>MIERGKFRSLTLVNWNGFFARTFDLDELVTTLSGGNGAGKSTTMAAFVTALIPDLTLLHFRNTTEAGATSGSRDKGLHGKLRAGVCYSTLDVINSRHQRVVVGVRLQQVAGRDRKVDIKPFMIQGLPTAIQPTQLLTENVGERQARVLPLNELKDRLDEMEGVQFKQFNSITDYHAQMFDLGVIPKRLRSASDRSKFYRLIEASLYGGISSAITRSLRDYLLPENSGVRKAFQDMEAALRENRITLEAIRVTQSDRDLFKHLITEATSYVSADYMRHANERRTHLDEALALRGELFGSHKQLATEQYRHVEMARELAEQSGASSDLETDHQAASDHLNLVQTAMRQQEKIDRYQVDLEELSYRLEEQTDVVEEAGELQAEYEARTEATEQEVDELKSQLADYQQALDVQQTRAIQYQQALQALERARELCRLPDLSVDNAEEWLETFQAKEQQATEALLALEQKLSVADAAHNQFEQAYQLVKNIVGETSRSEAWQSARELLRDWPSQRHLADRVQPLRMRLSELEQRLNNQQNAERLLSEFCKRQGRQYQAEDLEALQNELEARQEALSLSVNEGGERRMEMRQELEQLKQKIQSLTARAPVWLAAQDTLNQLCEQSGETLASSNDVTEYMQQLLEREREATVERDEVAAQKRELEKQIERLSQPSGAEDSRMIALAERFGGVLLSEIYDDITIDDAPYFSALYGPARHGIVVPDLSLVRPHLETLEDCPEDLYLIEGDPQSFDDSVFNAEEQTNAVLVKSSDRQWRYSRYPELPLFGRAARENRLEALNLERDALAERYATLSFDVQKIQRAHQAFSQFVGKHLSVAFDTDPEAEIRELRQRHTELEREVSRFEDQTQQQRQQYAQAKESLTTLNRLIPQVTLLLDETLIDRVEEVREEMDEAQEAARFLQQHGSALTKLEPMVAVLQSDPQQHEQLQQDYETAKHSQHQAKQQAFALVEIVQRRVHFSYSDSAGMLSENADLNDKLRQRLEHAESDRSRAREQLRQQQAQYSQFNQVLASLKSSYETKQDMLKELLQEMKDIGVQADANAEMRARERRDRLHEALSVNRSRVNQLEKQIAFCEAEMENVQKKLRKLERDYYQIREQVVSAKAGWCAVMRMVKDNGVERRLHRRELAYMEGGALRSMSDKALGALRLAVADNEHLRDALRLSEDPKRPERKVQFFIAVYQHLRERIRQDIIRTDDPVDAIEQMEIELARLTEELTAREQKLAISSKSVANIIRKTIQREQNRIRMLNQGLQAVSFGQVRGVRLNVNVRESHAILLDVLSEQQEQHQDLFNSQRLTFSEAMAKLYQRLNPQVDMGQRLPQTIGEELLDYRNYLELDVEVNRGSDGWLKAESGALSTGEAIGTGMSILVMVVQSWEEESRRLRGKDISPCRLLFLDEAARLDAKSIATLFELCERLQMQLIIAAPENISPEKGTTYKLVRKVFKNHEHVHVVGLRGFGQDAPATQLISDVTA[2x];>MSEYSQTVPELVSWARKNDFSISLPVERLAFLMAIAVLNSERLDGEMSEGELIDAFREVCKGFEQTAESVAVRANNAINDMVRQKLLNRFTSELADGNAIYRLTPLGISISDYYIRQREFSTLRLSMQLSIVANELHRAAEAAEEGGDEFHWHRNVFAPLKYSVAEIFDSIDMSQRLMDEQQNFVKEDIAALLNQDWQAAIANCEQLLSETSGTLRELQDTLEAAGDKLQANLLRIQDANMGSGGSELVDKLVFDLQSKLDRIISWGQQAIDLWIGYDRHVHKFIRTAIDMDKNRIFSQRLRQSVQHYFDNPWTLTVANAERLLDMRDEELALRNEEVTGELPLELEYEEFSEINDQLAAMIEKALLVYQQEQRPLDLGAVLRDYLAQHPLPRHFDVARILVDQAVRLGVAEADFSGLPAEWLAINDYGAKVQAHVIDTY[2x];>MSSTHIEQFMPVKLAQALANSLFPELDSQLRAGRHIGIDDLDNHAFLMDFQEQLEEFYARYNVELIRAPEGFFYLRPRSTTLIPRSVLSELDMMVGKILCYLYLSPERLANQGIFTSQELYEELISLADEGKLMKFVNQRSSGSDLDKQKLQEKVRTTLNRLRRLGMVYFLPNNNNKFTITEAVFRFGADVRSGDDPREIQLRMIRDGEAMPVEGSLSLDDSENDETPDNSAEGAGDEQP[2x];>[2x]MSTIEERVKKIIGEQLGVKQEEVTNNASFVEDLGADXLDTVELVMALEEEFDTEIPDEEAEKITTVQAAIDYINGHQA

MukBEF folds the chromosome of Escherichia coli and related bacteria. The SMC protein MukB dimerizes at its ‘‘hinge’’ domain, which connects via the long coiled-coil ‘‘arm’’ to the ABC-type ATPase ‘‘head’’ domain. The heads are bridged by the kleisin MukF, whereby the C-terminal winged-helix domain (cWHD) of MukF binds the ‘‘cap’’ surface of one MukB, and the N-terminal middle domain (MD) binds the coiled-coil ‘‘neck’’ of the other MukB. MukF also recruits the dimeric KITE protein MukE.

Using cryoelectron microscopy (cryo-EM), we demonstrate that ATP binding opens one of MukBEF’s three potential DNA entry gates, exposing a DNA capture site that positions DNA at the open neck gate. All three conditions enabled the reconstruction of a state with engaged heads, and we pooled the datasets to increase the signal and obtain higher resolution (STAR Methods). The resolved state was free of DNA, and the neck gate had opened widely. The neck and head regions of MukB adopted radically different conformations from what we had previously observed for the apo and DNA-bound unloading states of MukBEF. ATP binding and head engagement had triggered the detachment of the MukF MD from the MukB neck, which resulted in a swing-out of the MD of about 180°. Detachment of the MD was facilitated by the mechanical distortion of the MukB neck constrained between engaged heads and aligned arms, while the MD swing-out was stabilized by the binding of MukE to the top surface of the heads. This surface is formed by the engagement of the heads upon ATP binding and is a highly conserved DNA-binding site in all SMC complexes. Our structure reveals that occupation of the top of the heads by MukE and DNA is mutually exclusive, suggesting that MukE senses the DNA-free state of the heads to open the neck gate. Our findings show that MukBEF employs a dedicated mechanism for opening its neck gate, converting the DNA-free apo form to the open-gate state: (1) ATP binds the heads and leads to their engagement, (2) the neck distorts and releases the MD of MukF, (3) MukE binds the DNA-free top of the heads and stabilizes the open-gate state. This mechanism ensures that the gate opens only when the heads are DNA-free, which serves as an indicator that the complex is ready for loading.>MFEKLYSAIIYSDEFKKILLGRGVDDLEIASAYIAFLYEDLPIIGKNLCAAFLRMGLDAVYNVMPSGKVYSPRHKLYPISRYGIDGVCINCDGGKIILRISNKGYDPEDLLESKGLESRIFVSKNFKKKSMEIIEKIWDVNKIRLIARKEILERISAGGILHMIRLEHHHHH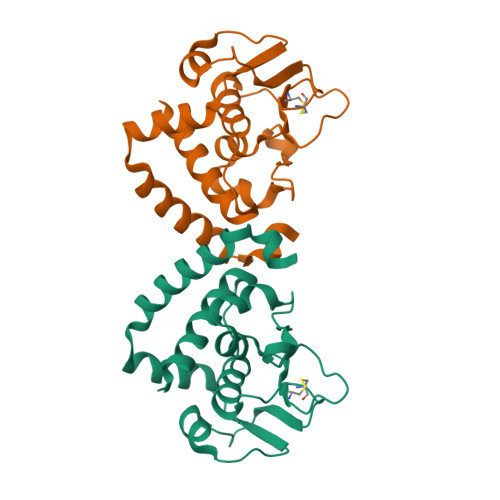H[4x]> MSEKMVAIMKTKPGYGAELVEVDVPKPGPGEVLIKV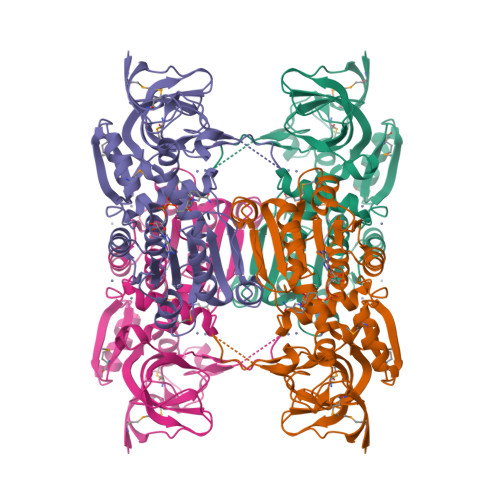LATSICGTDLHIYEWNEWAQSRIKPPQIMGHEVAGEVVEIGPGVEGIEVGDYVSVETHIVCGKCYACRRGQYHVCQNTKIFGVDTDGVFAEYAVVPAQNIWKNPKSIPPEYATLQEPLGNAVDTVLAGPISGKSVLITGAGPLGLLGIAVAKASGAYPVIVSEPSDFRRELAKKVGADYVINPFEEDVVKEVMDITDGNGVDVFLEFSGAPKALEQGLQAVTPAGRVSLLGLYPGKVTIDFNNLIIFKALTIYGITGRHLWETWYTVSRLLQSGKLNLDPIITHKYKGFDKYEEAFELMRAGKTGKVVFMLK Amicoumacin A | C20 H29 N3 O7 | 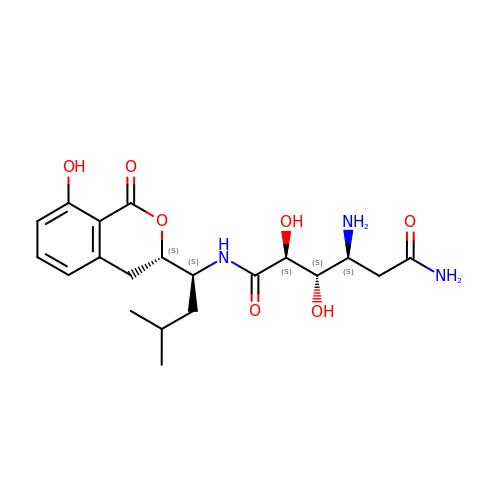DCPWYLSPIAHJFU-YKRRISCLSA-N> GAMEVIKNPKVFIDPLSVFKEIPFREDILRDAAIAIRYFVKNEVKFSNLFLGLTGTGKTFVSKYIFNEIEEVKKEDEEYKDVKQAYVNCREVGG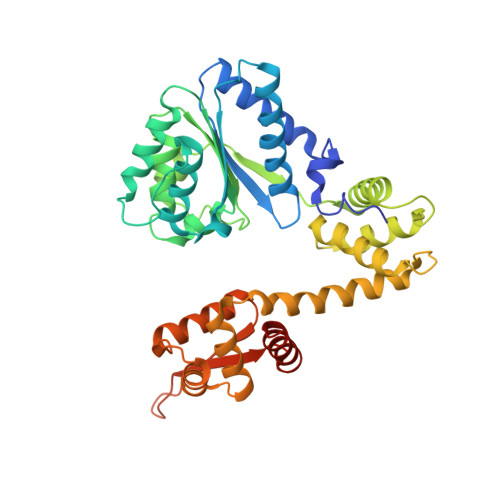TPQAVLSSLAGKLTGFSVPKHGINLGEYIDKIKNGTRNIRAIIYLDEVDTLVKRRGGDIVLYQLLRSDANISVIMISNDINVRDYMEPRVLSSLGPSVIFKPYDAEQLKFILSKYAEYGLIKGTYDDEILSYIAAISAKEHGDARKAVNLLFRAAQLASGGGIIRKEHVDKAIVDYEQERLIEAVKALPFHYKLALRSLIESEDVMSAHKMYTDLCNKFKQKPLSYRRFSDIISELDMFGIVKIRIINRGRAGGVKKYALVEDKEKVLRALNETFEDSISIGDFDDVGEN>MRKIGIIGGTFDPPHYGHLLIANEVYHALNLEEVWFLPNQIPPHKQGRDITSVESRLQMLELATEAEEHFSICLEELSRKGPSYTYDTMLQLTKKYPDVQFHFIIGGDMVEYLPKWYNIEALLDLVTFVGVARPGYKLRTPYPITTVEIPEFAVSSSLLRERYKE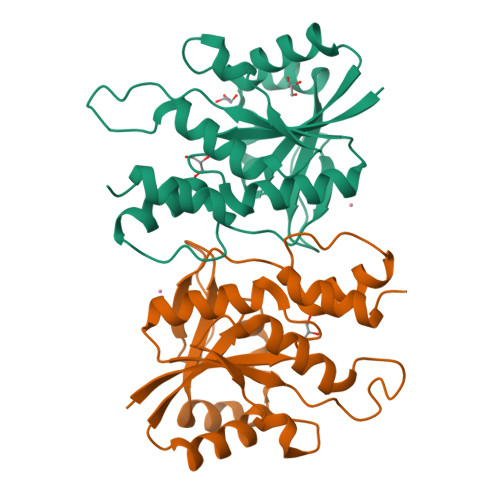KKTCKYLLPEKVQVYIERNGLYES[2x]> METPIAEELAKKQKSISVAEFFEKNRQILGFDSAPRSLITTVKEAVDNALDACEEAGILPDILVQVERTGPDYVTVIIEDNGPGIVREQIPKVFAKLLYGSRFHALKQSRGQQGIGISAAVLYAQMTAGRHTKILSKTSPTAPAHYYELMINTSTNEPDILVDEVRDWFRPHGTQIELEMRAAYVKGRRQSIYEYLKATAIVNPHARITLIDPDGNEEVFERATDKMPEPAEEILPHPEGIELGTLMKMLHYTERQKLAPFLRYSFCKIGLLTAEEICKAAGLDPEIDPHALGRHEARKLIEAFEKVKIMAPPTD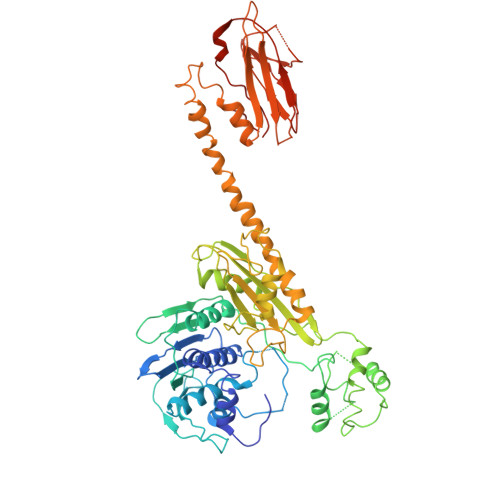CLSPIGEDLIYRGLEKETTVDFIATSTRKPAVYSGNPFVVEVGMAYGGNLPKEEKISIMRFANRVPLLYQQGGCVTTHAVEDIKWKQYGLNQPGGGIPVGPVILLIHVASINVPFTSESKDAIADIPVIKEEIDLAIKEVARKLKHYLSKQSNLKKRREKEIIITKVLPKLAAKVAHVLEKDVPDINPVVAKIMGNLLVHRVIKNNGDGTVDVAIKVKNFGTSAYSFRVHEMLPCKVSGAKPEPKVVTMGNDYDYVWDISASAGSSKVLSYKIESASEEELQKLPQLIVEGIEEELVTGAKAFKGV In all of these systems, the Fe-S cluster is formed on a scaffold protein before it is transferred to a target apoprotein. A cysteine desulfurase acquires sulfur from cysteine in a pyrodoxal-5ʹ-phosphate (PLP)-dependent reaction and then transfers it as persulfide to the scaffold protein. However, only the product of the sufS gene is involved in biosynthesis of Fe-S clusters. BsSufS assumes a type I fold of the aminotransferase class V family, consisting of an overall α/β fold that is highly similar to that of E. coli SufS, IscS, NifS, and CsdA.

We were able to determine the crystal structure of the BsSufS dimer to 1.7 Å resolution, revealing high structural homology to its E. coli counterpart. One molecule of SufS was found within the asymmetric unit (AU) and could be built to completeness. The BsSufS monomer forms a tightly intertwined homodimer with another monomer across the crystallographic symmetry axis. The interface and architecture of the BsSufS homodimer closely resemble those of E. coli SufS. The enzyme consists of two domains: A large, N-terminal domain (residues 1–294) and a smaller, C-terminal domain (residues 295–406). In the N-terminal domain, a 7-stranded, parallel β-sheet is sandwiched between several α-helices to form a tightly packed core. This domain harbors the active site pocket, where the cofactor PLP is bound to Lys224 as an aldimine. Furthermore, residues 253–265 (herein referred to as the ‘β-hook’) form a hairpin-like structure that latches on to the other monomer. The small, C-terminal domain consists of a 4-stranded, parallel β-sheet and four α-helices containing the flexible ‘Cys361-loop’ with the nucleophile Cys361. We found BsSufS in the product-bound state, with alanine bound near Cys361-persulfide, suggesting that one reaction cycle had occurred.

> MNITDIREQFPILHQQVNGHDLVYLDSAATSQKPRAVIETLDKYYNQYNSNVHRGVHTLGTRATDGYEGAREKVRKFINAKSMAEIIFTKGTTTSLNMVALSYARANLKPGDEVVITYMEHHANIIPWQQAVKATGATLKYIPLQEDGTISLEDVRETVTSNTKIVAVSHVSNVLGTVNPIKEMAKIAHDNGAVIVVDGAQSTPHMKIDVQDLDCDFFALSSHKMCGPTGVGVLYGKKALLENMEPAEFGGEMIDFVGLYESTWKELPWKFEAGTPIIAGAIGLGAAIDFLEEIGLDEISRHEHKLAAYALERFRQLDGVTVYGPEERAGLVTFNLDDVHPHDVATVLDAEGIAVRAGHHCAQPLMKWLDVTATARASFYLYNTEEEIDKLVEALQKTKEYFTNVFSGHHHHHH(1S,2R,3R,4S,6S)-6-[(8-azidooctanoyl)amino]-2,3,4-trihydroxycyclohexane-1-carboxylate | 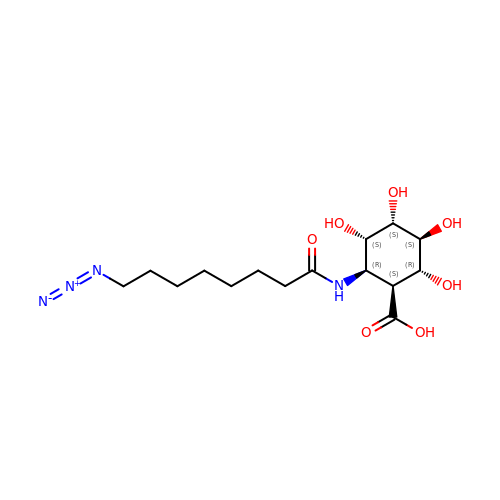C15 H26 N4 O7 | BTDXZNFDEBZDRR-KTEZLCCFSA-N> MSGSEEEKPIVIDLNKTIERDGRKVKLVRATITVDPETNTITIDIEYEGGPITKEDLLEAFKLAASKLGS

Here we use deep network hallucination to generate a wide range of symmetric protein homo-oligomers given only a specification of the number of protomers and the protomer length. Starting from only a choice of chain length L and oligomer valency N (2 for a dimer, 3 for a trimer, etc.), the method carries out a Monte Carlo search in sequence space starting from a random sequence. The loss function guiding the search is computed by inputting N copies of the sequence into the AlphaFold2 (AF2) network, and combining structure prediction confidence metrics (pLDDT; per-residue structural accuracy, and pTM; an estimate of the TM-score) with a measure of cyclic symmetry (the standard deviation of the distances between the center of mass of adjacent protomers within the predicted structure). To eliminate such over-fitting, we generated new sequences for the HAL backbones using the recently developed ProteinMPNN sequence design neural network (accompanying manuscript: Dauparas et al.).

To evaluate design accuracy we attempted crystallization of 19 designs and succeeded in solving crystal structures for seven (three C2s, two C3s and two C4s). All crystal structures had the correct oligomerization state and closely matched the design models (median Cα RMSD of 0.6 Å across all designs, with resolutions ranging from 1.8 to 3.4 Å). The side chain conformations in the crystal structures also closely match those of the design models. HALC2_062 is a three-layer homo-dimer with a single helix from each protomer packed together between two outer β-sheets (one from each protomer), while HALC2_065 is also a mixed α/β homo-dimer, but has a single, continuous β-sheet shared between both chains, which wraps around two perpendicular paired helices. These two hallucinated structures are distinct from any structure in the PDB, with TM-scores to their best matches of 0.59 and 0.54 respectively.>MAHHHHHHSSGLEVLFQGPMAQRRPAGKKIPFQKDSFLQQFEKLAQSRKHHVLLESARGGRYSIAGLDPIATVKGKDGITTIKHGDEMLFKEGDPLRAFHSWFKTLETETNHEFPDFQGGAIGFLSYDYARYIENFKMLSLDDLETPDIYFLVFDDIAVYDHQEESLWLITHVNGSDQETADVKLSELEQMWLTELPAVTSREMKPETAGSFAAPFTEDGFSQAVEKIKQYIASGDVFQVNLSIRQSQSLSVHPYQIYKTLREVNPSPYMAYLETPDFQIICGSPELLVSKKGKLLETRPIAGTRSRGKTNEEDEALANELIHNEKERAEHVMLVDLERNDLGRVSRYGSVRVNEFMAIEKYSHVMHIVSNVQGELQDGY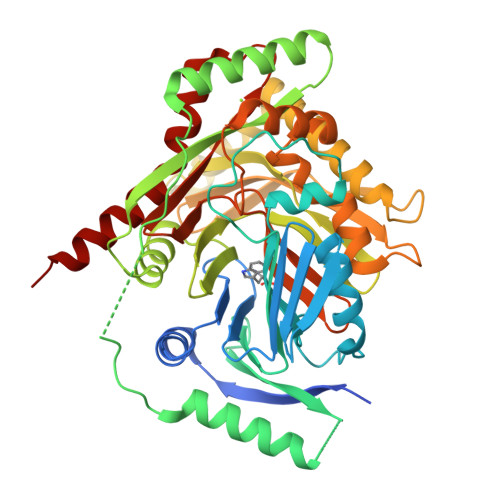DAVDIIHAVFPGGTITGAPKVRTMEIIEELEPTRRGLYTGSIGWFGYNHDLQFNIVIRTIYATGGQAFMQSGAGVVIDSVPKHEYKESFKKAFAMQRALELSEEETKIR[4x]> GHM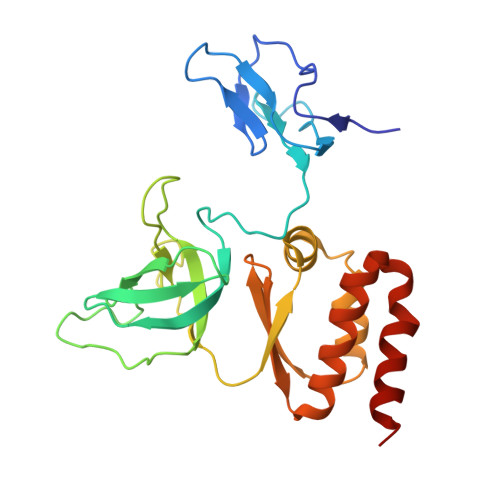STFIFPGDSFPVDPTTPVKLGPGIYCDPNTQEIRPVNTGVLHVSAKGKSGVQTAYIDYSSKRYIPSVNDFVIGVIIGTFSDSYKVSLQNFSSSVSLSYMAFPNASKKNRPTLQVGDLVYARVCTAEKELEAEIECFDSTTGRDAGFGILEDGMIIDVNLNFARQLLFNNDFPLLKVLAAHTKFEVAIGLNGKIWVKCEELSNTLACYRTIMECCQKNDTAAFKDIAKRQFKEILTVKEE>[2x]MGNMERDLFEKKFKEIKDKWVTDKQADEFIETADKYADKAVQMSAVASRAEYYRMYVSRKYHYKKEFVEKLKQVYKESGA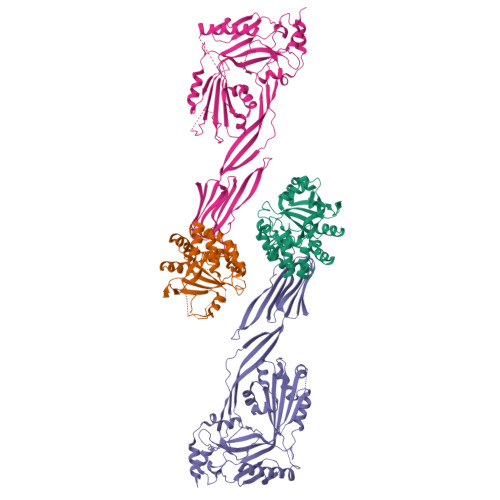SHVTSKKDLMLAFDDAKRKSTIGRQENGLFVTSFAEDMALLFTDQGKLKSADQIENIKDVDSGKYSDGVYQYEYDSELTKNIDKLGYIRTASGDTPRANSLNIPGCQTWSGKHIENSESELIFPSISVKDLKSKAVLAEIDAKGYFEIIDPTIIAPNGDHKKVTGRFKIKKMQDRMQDRKLEHHHHHH;>[2x]MASEDHTEEINDKIYSLNYNELEVLAKNGETIENFVPKEGVKKADKFIVIERKKKNINTTPVDISIIDSVTDRTYPAALQLANKGFTENKPDAVVTKRNPQKIHIDLPGMGDKATVEVNDPTYANVSTAIDNLVNQWHDNYSGGNTLPARTQYTESMVYSKSQIEAALNVNSKILDGTLGIDFKSISKGEKKVMIAAYKQIFYTVSANLPNNPADVFDKSVTFKELQRKGVSNEAPPLFVSNVAYGRTVFVKLETSSKSNDVEAAFSAALKGTDVKTNGKYSDILENSSFTAVVLGGDAAEHNKVVTKDFDVIRNVIKDNATFSRKNPAYPISYTSVFLKNNKIAGVNNRSEYVETTSTEYTSGKINLSHQGAYVAQYEILWDEINYDDKGKEVITKRRWDNNWYSKTSPFSTVIPLGANSRNIRIMARECTGLAWEWWRKVIDERDVKLSKEINVNISGSTLSPYGSITYK> MTTTERPDLAWLDEVTMTQLERNPYEVYERLRAEAPLAFVPVLGSYVASTAEVCREVATSPDFEAVITPAGGRTFGHPAIIGVNGDIHADLRSMVEPALQPAEVDRWIDDLVRPIARRYLERFENDGHAELVAQYCEPVSVRSLGDLLGLQEVDSDKLREWFAKLNRSFTNAAVDENGEFANPEGFAEGDQAKAEIRAVVDPLIDKWIEHPDDSAISHW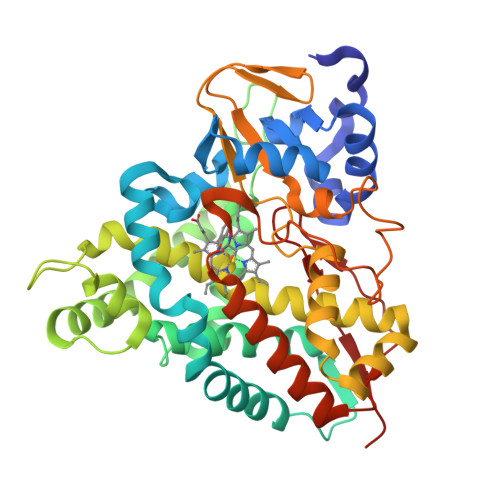LHDGMPPGQTRDREYIYPTIYVYLLGAMQEPGHGMASTLVGLFSRPEQLEEVVDDPTLIPRAIAEGLRWTSPIWSAGARISTKPVTIAGVDLPAGTPVMLSYGSANHDTGKYEAPSQYDLHRPPLPHLAFGAGNHACAGIYFANHVMRIALEELFEAIPNLERDTREGVEFWGWGFRGPTSLHVTWEV> MNHKVHHHHHHIEGRHMPLNNYLHVFYYSWYGNPQFDGKYIHWNHPVLEHWDPRIAKNYPQGRHNPPDDIGSSFYPELGSYSSRDPSVIETHMRQMRSASIGVLALSWYPPDVNDENGEPTDNLVPTILDKAHKYNLKVTFHIEPYSN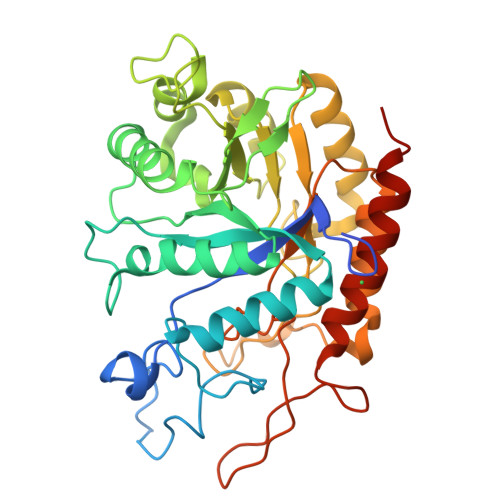RDDQNMYKNVKYIIDKYGNHPAFYRYKTKTGNALPMFYVYDSYITKPEKWANLLTTSGSRSIRNSPYDGLFIALLVEEKHKYDILQSGFDGIYTYFATNGFTYGSSHQNWASLKLFCDKYNLIFIPSVGPGYIDTSIRPWNTQNTRNRINGKYYEIGLSAALQTRPSLISITSFNEWHEGTQIEKAVPKRTSNTVYLDYRPHKPGLYLELTRKWSEKYSKERATYALDRQLPVS> MGLKLDLTWFDKSTEDFKGEEYSKDFGDDGSVMESLGVPFKDNVNNGCFDVIAEWVPLLQPYFNHQIDISDNEYFVSFDYRDGDW;> GFKDYGHDYHPAPKTENIKGLGDLKPGIPKTPKQNGGGKRKRWTGDKGR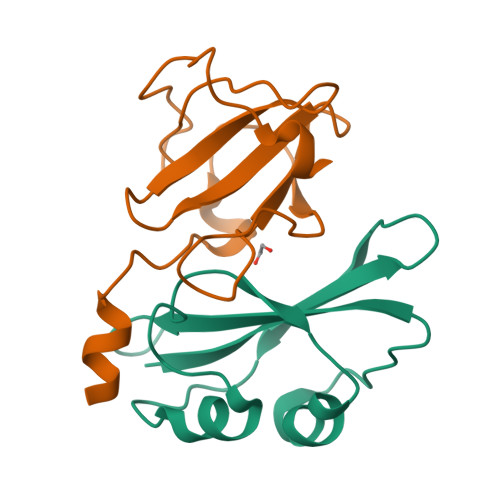KIYEWDSQHGELEGYRASDGQHLGSFDPKTGNQLKGPDPKRNIKKYL> DITVYNGQHKEAATAVAKAFEQETGIKVTLNSGKSEQLAGQLKEEGDKTPADVFYTEQTATFADLSEAGLLAPISEQTIQQTAQKGVPLAPKKDWIALSGRSRVVVYDHTKLSEKDMEKSVLDYATPKWKGKIGYVSTSGAFLEQVVALSKMKGDKVALNWLKGLKENGKLYAKNSVALQAVENGEVPAA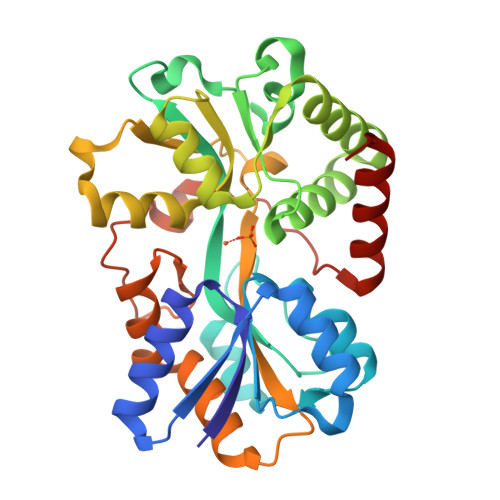LINNYYWYNLAKEKGVENLKSRLYFVRHQDPGALVSYSGAAVLKASKNQAEAQKFVDFLASKKGQEALVAARAEYPLRADVVSPFNLEPYEKLEAPVVSATTAQDKEHAIKLIEEAGLK>LKCNKLVP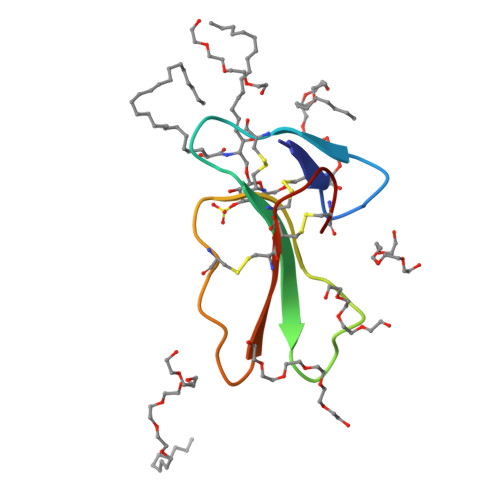LFYKTCPAGKNLCYKMFMVATPKVPVKRGCIDVCPKSSLLVKYVCCNTDRCN[2x]> ERVNVNLTSIKKLREKVDDSIHRELTDIFANLNYVGVVDEERRLAAIQHDLKLFLIDYGSVCYELFYQIGLTDFANFGKINLQSTNVSDDIVLYNLLSEFDELNDDASKEKIISKIWDMSSMLNEYYSIELVNDGLDNDLKSVKLKSLPLLLKGYIPSLVKLPFFIYRLGKEVDWEDEQECLDGILREIALLYIPDMVPKVDTSDASLSEDEKAQFINRKEHIS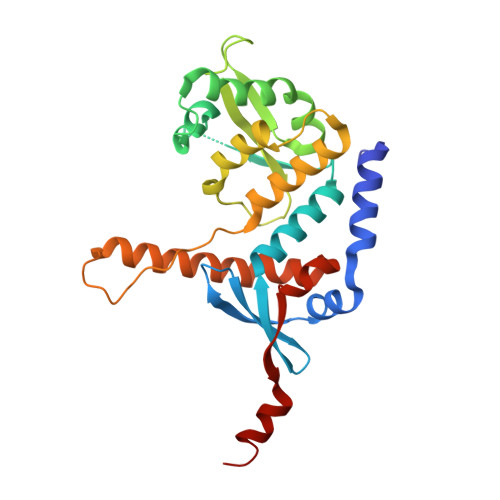SLLEHVLFPCIKRRFLAPRHILKDVVEIANLPDLYKVFERC> X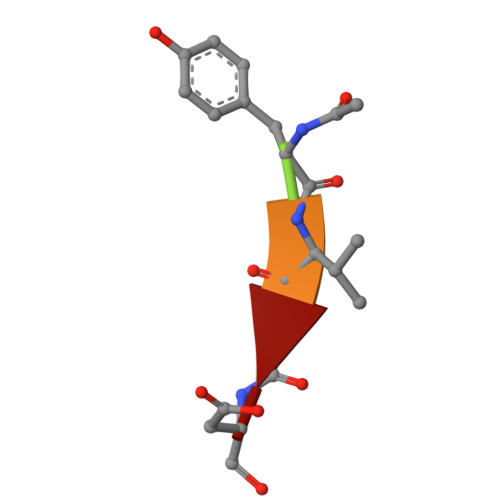YVAD>MSLHASAIESIETIIVDLPTIRPHKLAMHTMQNQTLVLIRLRCADGIEGLGESTTIGGLAYGNESPDSIKTNIDRFVAPLLIGQDASNINAAMLRLEQSIRGNTFAKSGIESALLDAQGKRLGLPVSELLGGRVRDALPVAWTLASGDTAKDIAEAQKMLDLRRHRIFKLKIGAGEVDRDLAHVIAIKKALGDSASVRVDVNQAWDEAVALRACRILGGNGIDLIEQPISRNNRAGMVRLNASSPAPIMADESIECVEDAFNLAREGAASVFAL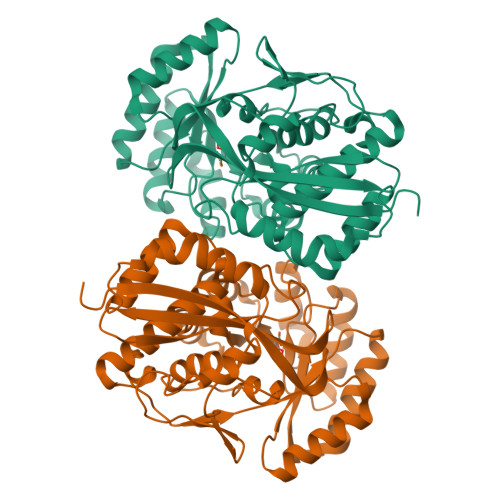KIAKNGGPRATLRTAAIAEAAGIGLYGGTMLEGGIGTLASAHAFLTLNKLSWDTELFGPLLLTEDILAEPPVYRDFHLHVSKAPGLGLSLDEERLAFFRREGHHHHHH[2x]>PPGPPGPPGPPGPXGPRXPPGPPGPPGPPG[3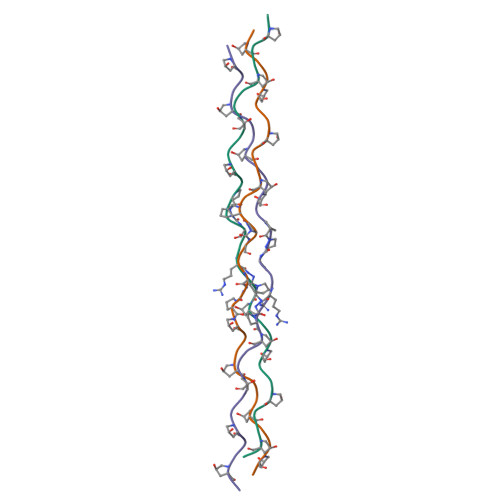x]>AESTLGAAAAQSGRYFGTAIASGKLGDSAYTTIASREFNMVTAENEMKIDATEPQRGQFNFSAGDRVYNWAVQNGKQVRGHALAWHSQQPGWMQSLSGSTLRQAMIDHINGVMGHYKGKIAQWDVVSHAFSDDGSGGRRDSNLQRTGNDWIEVAFRTARAADPAAKLCYNDYNIENWTWAKTQGVYNMVRDFKQRGVPIDCVGFQSHFNSGSPYNSNFRTTLQNFAALGVDVAITELDIQGASSSTYAAVTNDCLAVSRCLGITVWGVRDTDSWRSGDTPLLFNGDGSKKAAYTAVLNALNGGSSTPPPSGGGQIKGVGSGRCLDVPNASTTDGTQVQLYDCHSATNQQWTYTDAGELRVYGDKCLDAAGTGNGTKVQIYSCWGGDNQKWRLNSDGSIVGVQSGLCLDAVGGGTANGTLIQLYSCSNGSNQRWTRT[2x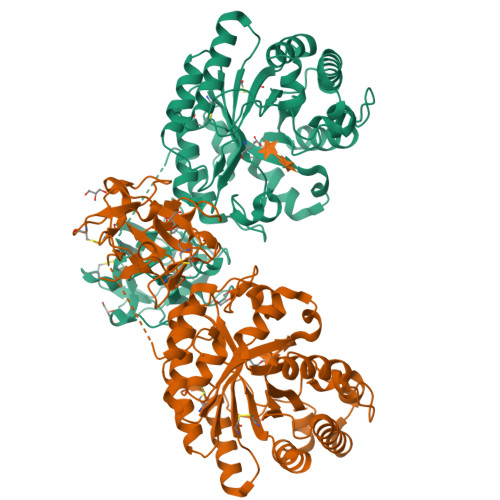]> MMINTQEDKLVSAHDAEEFHRFYIVQDDALLQEVNTLLTREAHLLDIQAYKAWLEHCVAPEIKYQVISRELRSTSERRYQLNDAVNIYNENYQQLKVRVEHQMDPQNWPNSPKIRFTRFVTNVTA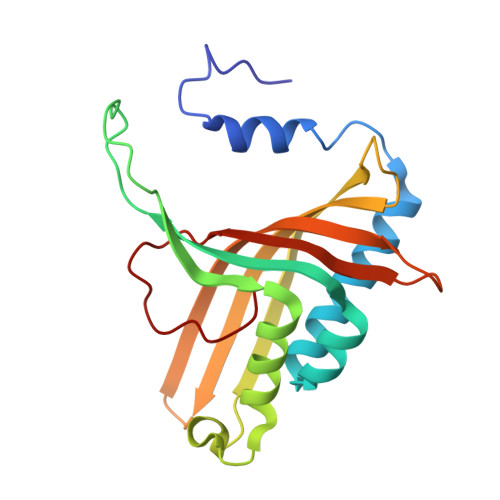AKDKSAPEMLHVRSNLILHRARRGNEVDVFYATREDKWKRIEGGGIQLVERFVDYPERILPHNLLVFL>NSLFNQEVQIPLTESYCGPCPKNWICYKNNCYQFFDESKNWYESQASCMSQNASLLKVYSKEDQDLLKLVKSYHWMGLVHIPTNGSWQWEDGSILSPNLLTIIEMQKGDCALYASSFKGYIENCSTPNTYICMQRTV[2x];> MEPHSLRYNLTVLSWDGSVQSGFLTEVHLDGQPFLRCDRQKCRAKPQGQWAEDVLGNKTWDRETRDLTGNGKDLRMTLAHIKDQKEGLHSLQEIRVCEIHEDNSTRSSQHFYYDGELFLSQNLETKEWTMPQSSRAQTLAMNVRNFLKEDAMKTKTHYHAMHADCLQELRRYLKSGVVLRRTVPPMVNVTRSEASEGNITVTC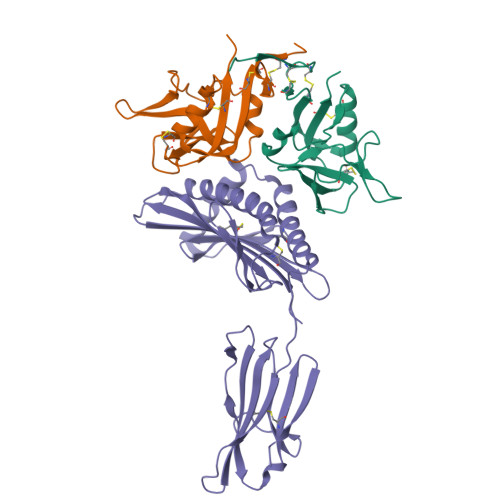RASGFYPWNITLSWRQDGVSLSHDTQQWGDVLPDGNGTYQTWVATRICQGEEQRFTCYMEHSGNHSTHPVPS>[2x]EDKYTDKYDNINLDEILANKRLLVAYVN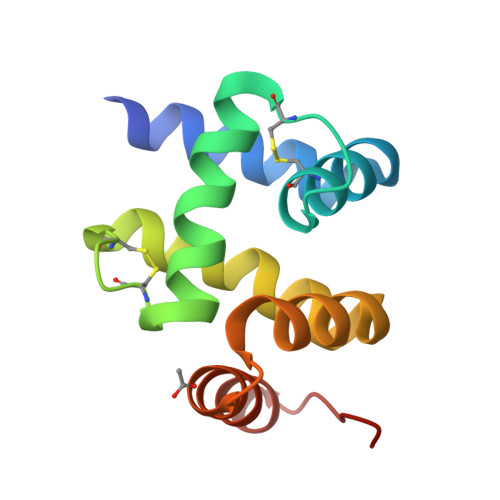CVMERGKCSPEGKELKEHLQDAIENGCKKCTENQEKGAYRVIEHLIKNEIEIWRELTAKYDPTGNWRKKYEDRAKAAGIVIPEE> CELDRDPEGKDFQQPYTSFVQTKQNRDGLYALLRNTENPRMHFYQELQSDMYCTTITDGNSLAPFVNWDLGILNDHGRADEDEVSGIAGYYFVYNRLNQQANAFVNNTEAALQNQVYKNSTEIANAKSFLAEGKVLQALAIWRLMDRFSFHESVTEVNSGAKDLGVILLKEYNPGYIGPRATKAQCYDYILSRLSEAIEVLPENRESVLYVSRDYAYALRARIYLALGEYGKAAADAKMVVDKYPLIGAADASEFENIYRSDAN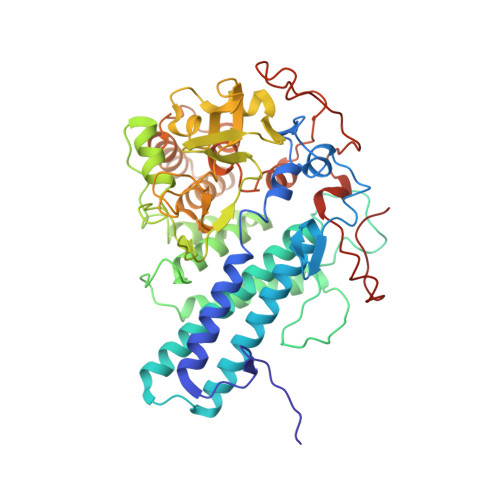NPEIIFRGFASATLGSFTATTLNGAAPAGKDIKYNPSAVPFQWVVDLYENEDFRKSVYIAKVVKKDKGYLVNKFLEDKAYRDVQDKPNLKVGARYFSVAEVYLILVESALQTGDTPTAEKYLKALSKARGAEVSVVNMEALQAERTRELIGEGSRLRDMVRWSIPNNHDAFETQPGLEGFANTTPLKAQAPVGFYAYTWEFPQRDRQTNPQLIKNWPI>[4x]GSHMGGWSIALHGGAGDIPFSLPPERRKPREEGLRHCLQIGVEALKAQKPPLDVVELVVRELENIEHFNAGIGSVLTNSGTVEMEASIMDGNTMKCGAVSGLSTVLNPI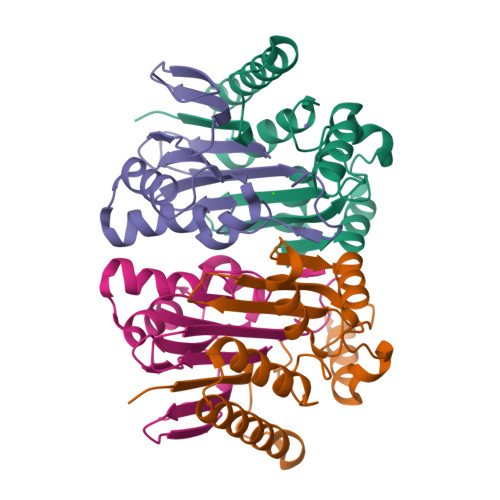SLARLVMDKTPHIYLAFQGAQDFAKQQGVETVDSSHLITAENVERLKLAIEANRVQVDYSQYNYPEPVKDDAEKELPLTNGDSQIG;>[4x]TVGCVAVDSHGNLASATSTGGLVNKMVGRIGDTPLIGAGTYANELCAVSATGKGEEIIRATVARDVAALMEFKGLSLKEAADFVIHERTPKGTVGLIAVSAAGEIAMPFNTTGMFRACATEDGYSEIAIWPTT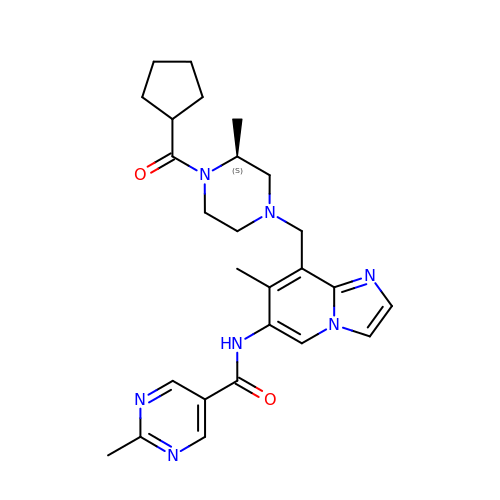~{N}-[8-[[(3~{S})-4-cyclopentylcarbonyl-3-methyl-piperazin-1-yl]methyl]-7-methyl-imidazo[1,2-a]pyridin-6-yl]-2-methyl-pyrimidine-5-carboxamide | C26 H33 N7 O2 | GMRCLEMCHGYDSY-KRWDZBQOSA-N> MKTFIIGISGVTNSGKTTLAKNLQKHLPNCSVISQDDFFKPESEIETDKNGFLQYDVLEALNMEKMMSAISCWMESARHSVVSTDQESAEEIPILIIEGFLLFNYKPLDTIWNRSYFLTIPYEECKRRRSTRVYQPPDSPGYFDGHVWPMYLKYRQEMQDITWEVVYLDGTKSE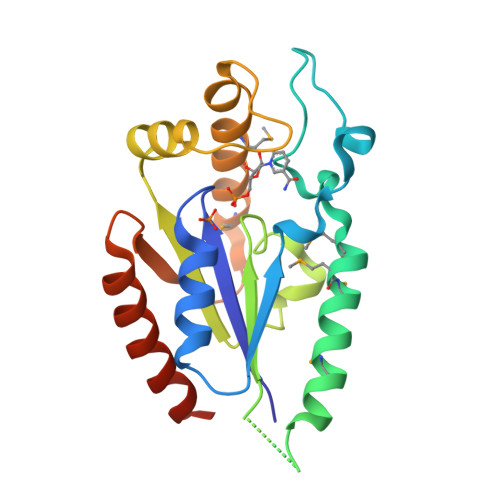EDLFLQVYEDLIQELAKQKCLQVTA>[2x]MQRGKVKWFNNEKGYGFIEVEGGSDVFVHFTAIQGEGFKTLEEGQEVSFEIVQGNRGP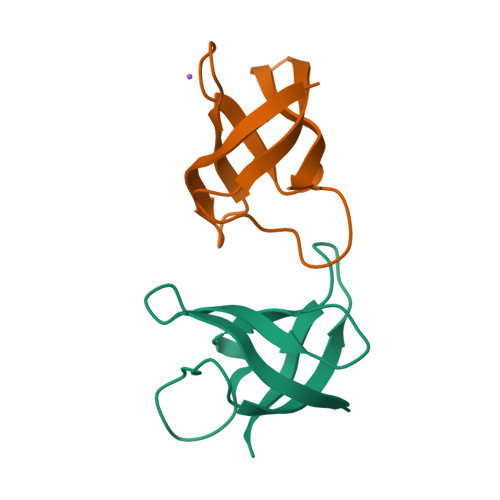QAANVVKE> SMACYGGFDLYFILDKSGSVLHHWNEIYYFVEQLAHKFISPQLRMSFIVFSTRGTTLMKLTEDREQIRQGLEELQKVLPGGDTYMHEGFERASEQIYYENRQGYRTASVIIALTDGELHEDLFFYSEREANRSRDLGAIVYAVGVKDFNETQLARIADSKDHVFPVNDGF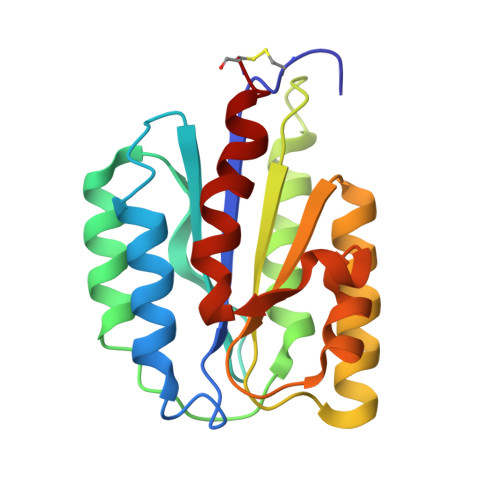QALQGIIHSILKKSC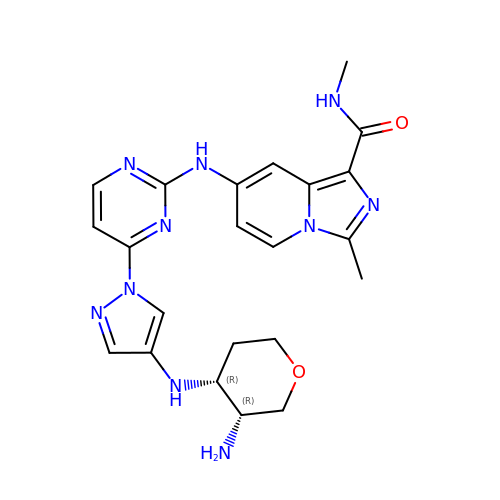7-[[4-[4-[[(3~{R},4~{R})-3-azanyloxan-4-yl]amino]pyrazol-1-yl]pyrimidin-2-yl]amino]-~{N},3-dimethyl-imidazo[1,5-a]pyridine-1-carboxamide | C22 H26 N10 O2 | OALOIHPPRINPBM-DLBZAZTESA-N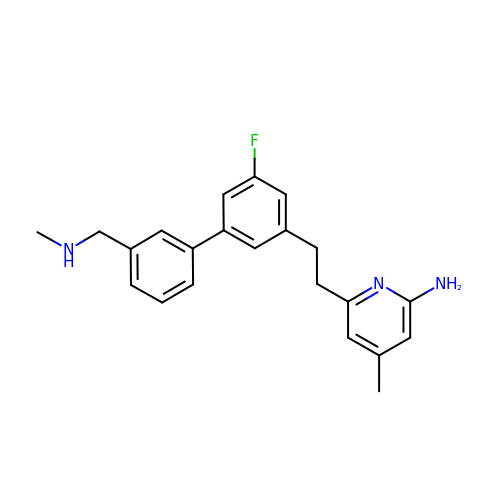6-(2-{5-fluoro-3'-[(methylamino)methyl][1,1'-biphenyl]-3-yl}ethyl)-4-methylpyridin-2-amine | C22 H24 F N3 | GVTRYBJMAVPTHT-UHFFFAOYSA-N>[5x]MAWDLKVK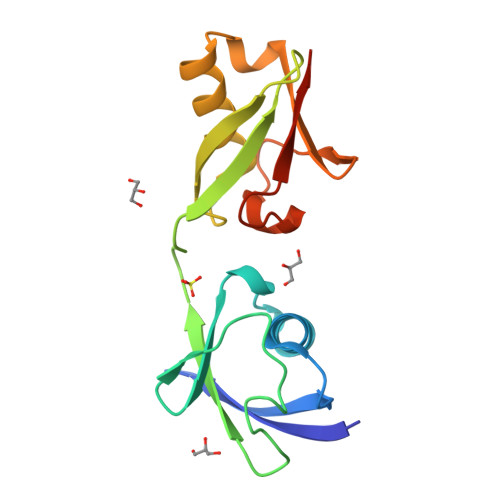MLGGNDFLVSVTNSMTVSELKKQIAQKIGVPAFQQRLAHQTAVLQDGLTLSSLGLGPSSTVMLVVQNSSEPLSILVRNERGHSNIYEVFLTQTVDTLKKKVSQREQVHEDQFWLSFEGRPMEDKELLGEYGLKPQCTVIKHLRLRGG> EVNXVAE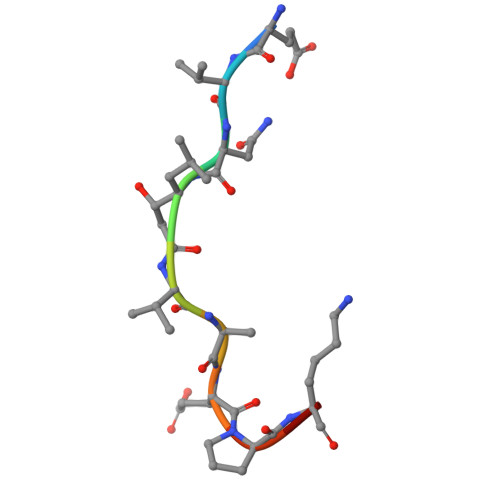PKX> MDVFQEGLAMVVQDPLLCDLPIQVTLEEVNSQIALEYGQAMTVRVCKMDGEVMPVVVVQSATVLDLKKAIQRYVQLKQEREGGIQHISWSYVWRTYHLTSAGEKLTEDRKKLRDYGIRNRDEVSFIKKLRQK;> MNDWMPIAKEYDPLKAGSIDGTDEDPHDRAVWRAMLARYVPNKGVIGDPLLTLFVARLNLQTKEDKLKEVFSRYGDIRRLRLVRDLVTGFSKGYAFIEYKEERAVIKAYRDADGLVIDQHEIFVDYELERTLKGWIPRRLGGGLGGKKESGQLRFGGRDRPFRKPINLPVVKNDLYREGKRERRERSRSRERHWDSRTRDRDHDRGREKRWQEREPTRVWPDNDWERERDFRDDRIKGREKKERGK;> MALPPFFGQGRPGPPPPQPPPPAPFGCPPPPLPSPAFPPPLPQRPGPFPGASAPFLQPPLALQPRASAEASRGGGGAGAFYPVPPPPLPPPPPQCRPFPGTDAGERPRPPPPGPGPPWSPRWPEAPPPPADVLGDAALQRLRDRQWLEA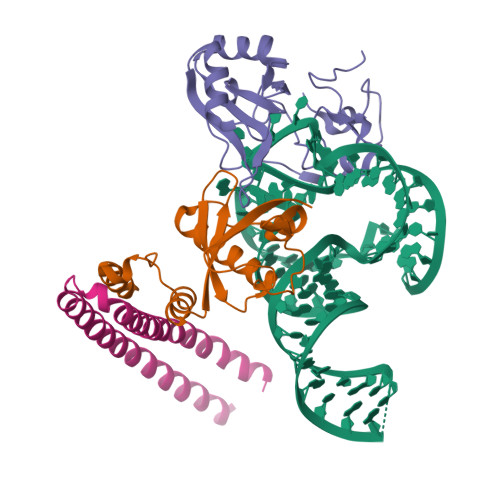VFGTPRRAGCPVPQRTHAGPSLGEVRARLLRALRLVRRLRGLSQALREAEADGAAWVLLYSQTAPLRAELAERLQPLTQAAYVGEARRRLERVRRRRLRLRERAREREAEREAEAARAVEREQEIDRWRVKCVQEVEEKKREQELKAAADGVLSEVRKKQADTKRMVDILRALEKLRKLRKEAAARKGVCPPASADETFTHHLQRLRKLIKKRSELYEAEERALRVMLEGEQEEERKRELEKKQRKEKEKILLQKREIESKLFGDPDEFPLAHLLEPFRQYYLQAEHSLPALIQIRHDWDQYLVPSDHPKGNFVPQGWVLPPLPSNDIWATAVKLH>TETTSFLITKFSPDQQNLIFQGDGYTTKEKLTLTKAVKNTVGRALYSSPIHIWDRETGNVANFVTSFTFVINAPNSYNVADGFTFFIAPVDTKPQTGGGYLGVFNSAEYDKTTQTVAVEFDTFYNAAWDPSNRDRHIGIDVNSIKSVNTKSWKLQNGEEANVVIAFNAATNV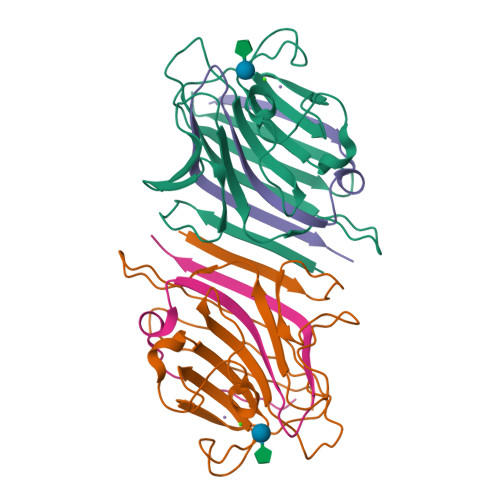LTVSLTYPNSLEEEN[2x];>VTSYTLSDVVSLKDVVPEWVRIGFSATTGAEYAAHEVLSWSFHSELSG[2x]2-[O-PHOSPHONOPYRIDOXYL]-AMINO- BUTYRIC ACID | C12 H19 N2 O7 P | 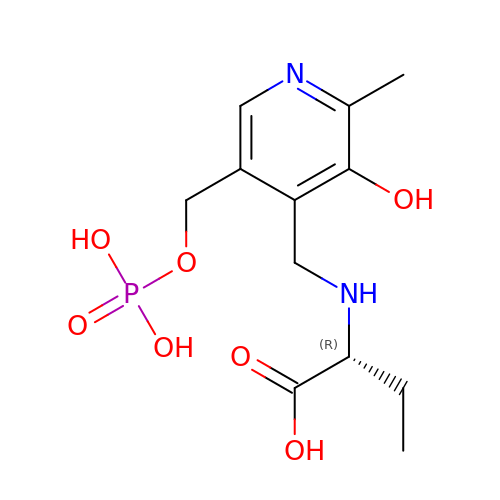VRMPGTOTVVJQMU-SNVBAGLBSA-N> SNKKTKLIHGGHTTDDYTGAVTTPIYQTSTYLQDDIGDLRQGYEYSRTANPTRSSVESVIATLENGKHGFAFSSGVAAISAVVMLLDKGDHIILNSDVYGGTNRALTKVFTRFGIEVDFVDTTHTDSIVQAIRPTTKMLFIETPSNPLLRVTD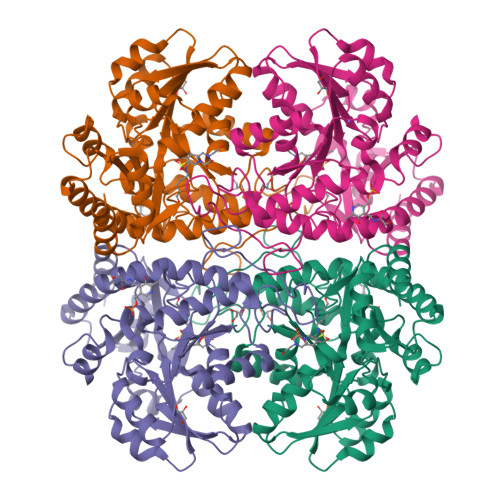IKKSAEIAKEHGLISVVDNTFMTPYYQNPLDLGIDIVLHSATKYLGGHSDVVAGLVATSDDKLAERLAFISNSTGGILGPQDSYLLVRGIKTLGLRMEQINRSVIEIIKMLQAHPAVQQVFHPSIESHLNHDVHMAQADGHTGVIAFEVKNTESAKQLIKATSYYTLAESLGAVESLISVPALMTHASIPADIRAKEGITDGLVRISVGIEDTEDLVDDLKQALDTL>[2x]GPLGSAKQQR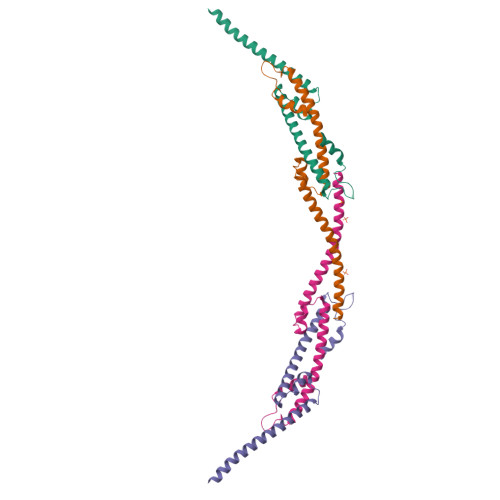AEATERVTAGLREVLAARERRAQLEAEGLANLKTLLKVVAVPATVAKTLDQARSAEEIADQVEILVDQTEKARELDVQAVAWLEHAQRTFETHPLSAASGDGPGLLTRQGARLQALFDTRRRVEALRR FabA, a homologue of FabZ, is an essential enzyme for Gram-negative bacteria. Unlike FabZ, FabA carries out a second enzymatic step, the isomerisation of (E)-2-enoyl-ACP to (Z)-3-enoyl-ACP (trans to cis C3–C4 double bond), an essential reaction to provide unsaturated fatty acids that are furthermore absent in eukaryotes. Further, unlike FabI, there are no isozymes of FabA. This makes FabA a particularly attractive target for drug discovery.

High-throughput screening of the PaFabA enzyme has discovered a new inhibitor, N42FTA, the first non-suicide inhibitor of this important and attractive target. To understand the mechanism of inhibition by N42FTA, we determined its co-crystal structure with PaFabA. N42FTA is bound at the active site formed by the two subunits of the canonical FabA dimer, and it bridges from the A subunit to the B subunit. Therefore, each dimer has two compounds bound. One nitrogen atom of the central triazole ring makes a hydrogen bond with main chain of A195 in the A subunit whilst the other two nitrogen atoms make hydrogen bonds to H70 and G79 in the B subunit. One water (W1), found in all five monomers in the asymmetric unit, bridges from the triazole to the side chain of D84 of the A subunit and the main chain of C80 of the B subunit. A second water (W2), which is absent in two monomers of the asymmetric unit, bridges the triazole ring and the amine of N42FTA to the key catalytic residues H70 of the B subunit and D84 of the A subunit. The chlorobenzene moiety makes very extensive van der Waal contacts filling the hydrophobic tunnel in the A subunit that binds the substrate acyl chain. These data suggest that N42FTA acts by blocking acyl chain substrate binding. Superposition of the N42FTA complex with the structure of H70N (inactive) PaFabA bound to 3-hydroxydecanoyl-NAC reveals that the triazole occupies the same volume as the thioester group of 3-hydroxydecanoyl-NAC.

>MTKQHAFTREDLLRCSRGELFGPGNAQLPAPNMLMIDRIVHISDVGGKYGKGELVAELDINPDLWFFACHFEGDPVMPGCLGLDAMWQLVGFYLGWQGNPGRGRALGSGEVKFFGQVLPTAKKVTYNIHIKRTINRSLVLAIADGTVSVDGREIYSAEGLRVGLFTSTDSF[5x]>[6x]ADECPTDWKMFNGRCFLFNPLQLHWADAQESCMKEGANLASIHSLEESTFVKELTSADLIPSWIGGTDCQVSTRWFWMDSTSMDYADWCAAQPDTTLTECCIQMNVGIGKCWNDTPCTHLHSSICAKPLKHHHHHH

Many species of ectothermic animals, plants, and microbes living in cold environments produce antifreeze proteins/polypeptides (AFPs) to protect them from freezing damage. AFPs can also inhibit ice recrystallization, of which the large ice crystals grow with the expense of smaller ones, thus prevent cell damages during freeze-thaw cycles. It is generally accepted that AFPs function through adsorption of their flat ice-binding surfaces onto particular planes of ice crystals and prevent or inhibit further ice growth. Type II AFPs are 14–24 kDa cysteine-rich proteins, which have been found in five fish species, including herring (Clupea harengus), rainbow smelt (Osmerus mordax), Japanese smelt (Hypomesus nipponensis), sea raven (Hemitripterus americanus) and longsnout poacher (Brachyopsis rostratus). They are the largest globular fish AFPs known to date, which are homologous to the C-type (Ca2+-dependent) lectin-like domains (CTLDs). Homology modeling and NMR studies on type II AFPs indicated that these proteins share the same characteristic fold, which includes disulfide bridges, α-helices and β-sheets, as well as a large proportion of coil structure. Both herring and two smelt AFPs depend on Ca2+ for their antifreeze activity, while the functions of sea raven and longsnout poacher AFPs are Ca2+ independent.

To understand the Ca2+-dependent ice-binding mechanism, we have determined the X-ray structure of the Ca2+-dependent type II hAFP at 1.7Å resolution. The crystal structure of hAFP, a first representative member of the Ca2+-dependent type II AFPs, has been determined. hAFP crystallized with six molecules in the asymmetric unit. Each hAFP monomer consists of residues from Cys4 to Lys130. Each monomer comprises two twisted anti-parallel β-sheets with an α-helix on either side. The overall three-dimensional fold of hAFP resembles the long-form CTLDs and is different from other types of AFPs. As expected, all 10 cysteines of hAFP are paired to form disulfide bonds, Cys4-Cys15, Cys32-Cys125, Cys69-Cys100, Cys89-Cys111 and Cys101-Cys117. Remarkably, the additional two disulfide bonds (Cys69-Cys100 and Cys89-Cys111) are located at each end of the Ca2+-binding loop (Gln92-Asp114). The bound Ca2+ is coordinated by Gln92 Oε1, Asp94 Oδ2, Glu99 Oε1, Asn113 Oδ1 and Asp114 O and Oδ1. The pentagonal bipyramidal coordinating sphere for Ca2+ is completed by a water molecule. Considering both the structural data and results of site-directed mutagenesis obtained here, together with the previous mutagenesis study of Ca2+-coordinating residues Asp94 and Glu99, which severely hampered the ice binding, we propose that the ice-binding site of hAFP consists of Asp94, Thr96, Thr98, and Glu99 that form a relatively flat surface to interact with ice.>MKKPRIDMHSHFFPRISEQEAAKFDANHAPWLQVSAKGDTGSIMMGKNNFRPVYQALWDPAFRIEEMDAQGVDVQVTCATPVMFGYTWEANKAAQWAERMNDFALEFAAHNPQRIKVLAQVPLQDLDLACKEASRAVAAGHLGIQIGNHLGDKDLDDATLEAFLTHCANEDIPILVHPWDMMGGQRMKKWMLPWLVAMPAET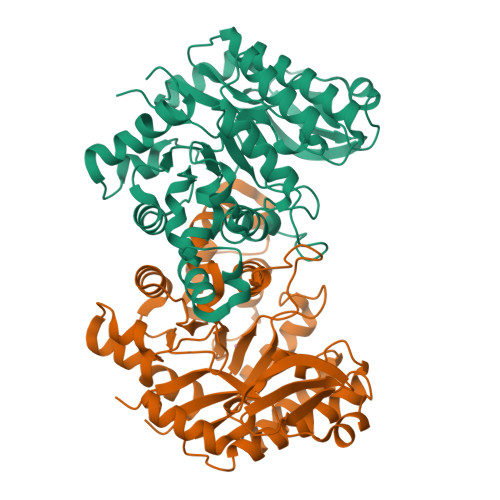QLAILSLILSGAFERIPKSLKICFGYGGGSFAFLLGRVDNAWRHRDIVREDCPRPPSEYVDRFFVDSAVFNPGALELLVSVMGEDRVMLGSDYPFPLGEQKIGGLVLSSNLGESAKDKIISGNASKFFNINV[2x]N,N-diethyl-4-methylbenzene-1-sulfonamide | C11 H17 N O2 S | 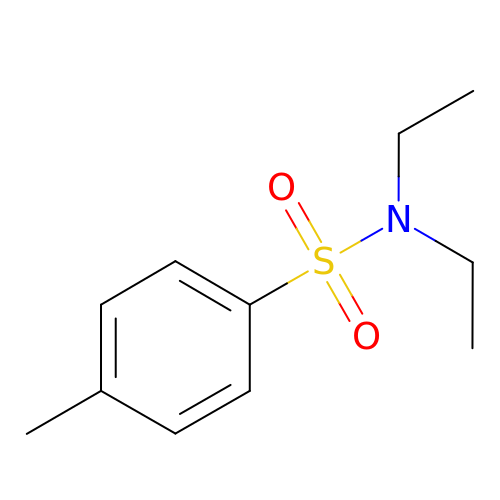AOJBACHWNDMRQP-UHFFFAOYSA-N>HHHHHHGSMTIPDVFPHLPLIAITRNPVFPRFIKIIEVKNKKLVELLRRKVRLAQPYVGVFLKRDDSNESDVVESLDEIYHTGTFAQIHEMQDLGDKLRMIVMGHRRVHISRQLEVEPEEPEAENKHKPRRKSKRGKKEAEDELSARHPAELAMEPTPELPAEVLMVEVENVVHEDFQVTEEVKALTAEIVKTIRDIIALNPLYRESVLQMMQAGQRVVDNPIYLSDMGAALTGAESHELQDVLEETNIPKRLYKALSLL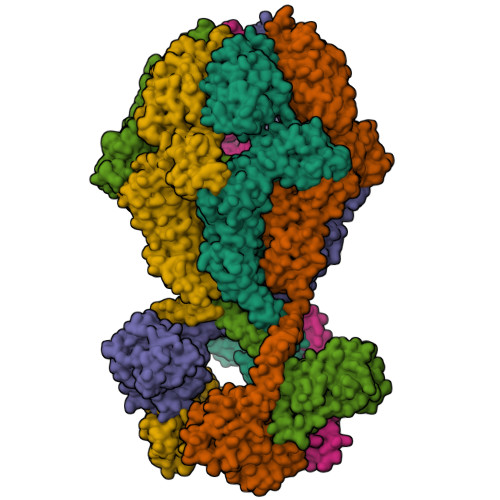KKEFELSKLQQRLGREVEEKIKQTHRKYLLQEQLKIIKKELGLEKDDKDAIEEKFRERLKELVVPKHVMDVVDEELSKLGLLDNHSSEFNVTRNYLDWLTSIPWGKYSNENLDLARAQAVLEEDHYGMEDVKKRILEFIAVSQLRGSTQGKILCFYGPPGVGKTSIARSIARALNREYFRFSVGGMTDVAEIKGHRRTYVGAMPGKIIQCLKKTKTENPLILIDEVDKIGRGYQGDPSSALLELLDPEQNANFLDHYLDVPVDLSKVLFICTANVTDTIPEPLRDRMEMINVSGYVAQEKLAIAERYLVPQARALCGLDESKAKLSSDVLTLLIKQYCRESGVRNLQKQVEKVLRKSAYKIVSGEAESVEVTPENLQDFVGKPVFTVERMYDVTPPGVVMGLAWTAMGGSTLFVETSLRRPQDKDAKGDKDGSLEVTGQLGEVMKESARIAYTFARAFLMQHAPANDYLVTSHIHLHVPEGATPKDGPSAGCTIVTALLSLAMGRPVRQNLAMTGEVSLTGKILPVGGIKEKTIAAKRAGVTCIVLPAENKKDFYDLAAFITEGLEVHFVEHYREIFDIAFPDEQAEALAVER[6x]>[2x]SKTKPFTLPILTLGELSNSRFPAPIDMLYTDPNEAIVVQPQNGRCTLDGTLQGTTQLVPTQICSFRGTLISQTSRSADSTDSAPRVRNHPLHVQLKNLDGTPYDPTDEVPAVLGAIDFKGTVFGVASQRNTTGNSIGATRAHEVHIDTTNPRYTPKLGSVLMYSESNDFDDGQPTRFTPIGMGADDWHQWELPEYSGHLTLNMNLAPAVAPAFPGERILFFRSVV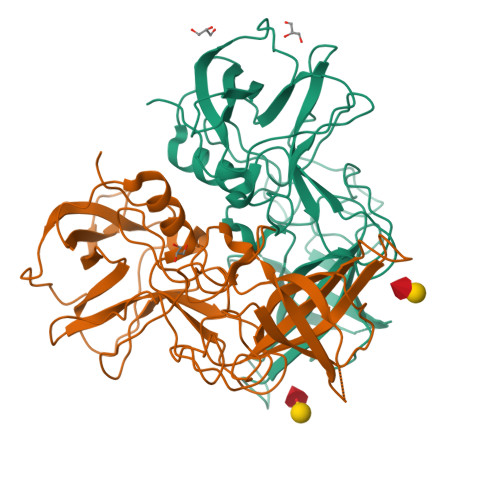PSAGGYGSGHIDCLIPQEWVQHFYQEAAPSQSAVALIRYVNPDTGRNIFEAKLHREGFITVANSGNNPIVVPPNGYFRFEAWVNQFYTLTPM> MDSGYSSSYAAAAGMHVVICPWLAFGALLPCLDLAQRLASRGHRVSFVSTPRNISRLPPVRPALAPLVAFVALPLPRVEGLPDGAESTNDVPHDRPDMVELHRRAFDGLAAPFSEFLGTACADWVIVDVFHHWAAAAALEHKVPCAMMLLGSAHMIASIADRRLERAETESPAAAGQGRPAAAPTFEVARMKLIRTKGSSGMS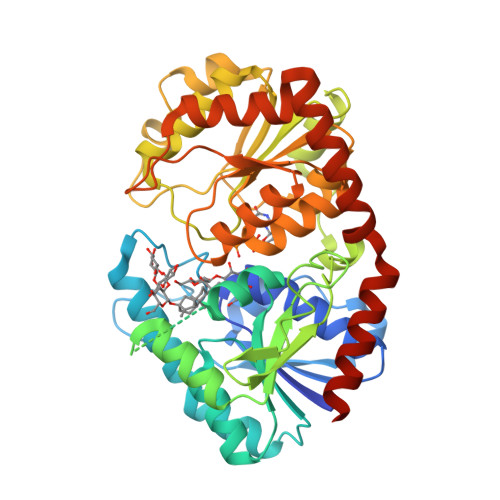LAERFSLTLSRSSLVVGRSCVEFEPETVPLLSTLRGKPITFLGLMPPLHEGRREDGEDATVRWLDAQPAKSVVYVALGSEVPLGVEKVHELALGLELAGTRFLWALRKPTGVSDADLLPAGFEERTRGRGVVATRWVPQMSILAHAAVGAFLTHCGWNSTIEGLMFGHPLIMLPIFGDQGPNARLIEAKNAGLQVARNDGDGSFDREGVAAAIRAVAVEEESSKVFQAKAKKLQEIVADMACHERYIDGFIQQLRSYKDLEHHHHHH>[2x]MSSRKELANAIRALSMDAVQKAKSGHPGAPMGMADIAEVLWRDFLKHNPQNPSWADRDRFVLSNGHGSMLIYSLLHLTGYDLPMEELKNFRQLHSKTPGHPEVGYTAGVETTTGPLGQGIANAVGMAIAEKTLAAQFNRPGHDIVDHYTYAFMGDGCMMEGISHEVCSLAGTLKLGKLIAFYDDNGISIDGHV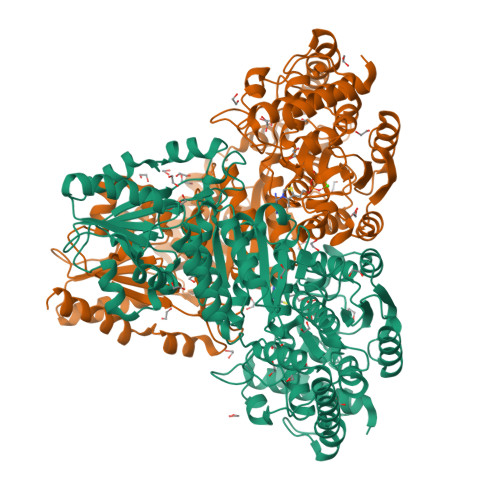EGWFTDDTAMRFEAYGWHVIRDIDGHDAASIKRAVEEARAVTDKPSLLMCKTIIGFGSPNKAGTHDSHGAPLGDAEIALTREQLGWKYAPFEIPSEIYAQWDAKEAGQAKESAWNEKFAAYAKAYPQEAAEFTRRMKGEMPSDFDAKAKEFIAKLQANPAKIASRKASQNAIEAFGPLLPEFLGGSADLAPYNLTLWSGSKAINEDAAGNYIHYGVREFGMTAIANGISLHGGFLPYTSTFLMFVEYARNAVRMAALMKQRQVMVYTHDSIGLGETGPTHQPVEQVASLRVTPNMSTWRPCDQVESAVAWKYGVERQDGPTALILSQQNLAQQERTEEQLANIARGGYVLKDCAGQPELIFIATGSEVELAVAAYEKLTAEGVKARVVSMPSTDAFDKQDAAYRESVLPKAVTARVAVEAGIADYWYKYVGLNGAIVGMTTFGESAPAELLFEEFGFTVDNVVAKAKELLHHHHHH> APSTTPVNEKATDAAKNLLSYLVEQAANGVTLSGQQDLESAQWVSDNVGKWPAILGIDFMDYSPSRVEYGAVGSTVPDAISYDSDGGIVTFCWHWGSPSGTYNTTDQPWWSNFYTEATAFDIAAAMDDPDSADYNL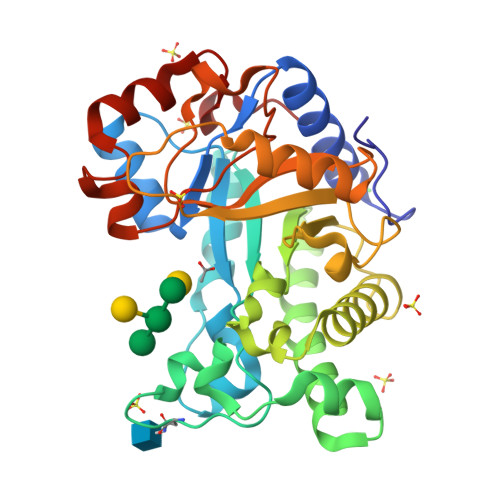LVRDIDAISELLLQLQDLDIPILWRPLHQAEGGWFWWGAKGPEACIALYRLMFDRMTNHHGLNNLLWVWNSVDPSWYPGNDVVDIVSADIYADAGDHSPQEETFASLQSLTGDTKLVALGEVGNIPDPASTGGVADWAYWVTWNGDFIKGEDYNPLEYKKEVFSAENIITRDEVDV(2R)-2-methyl-N-(phenylmethyl)-3-sulfanyl-propanamide 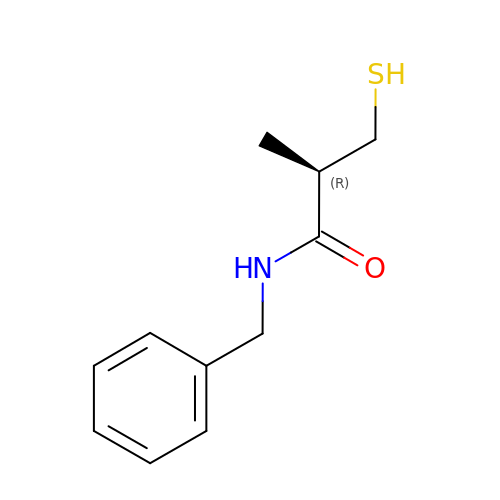| C11 H15 N O S | OOFLQSFFPITNLC-VIFPVBQESA-N2-(1H-INDOL-3-YL)ETHANIMINE | C10 H10 N2 | 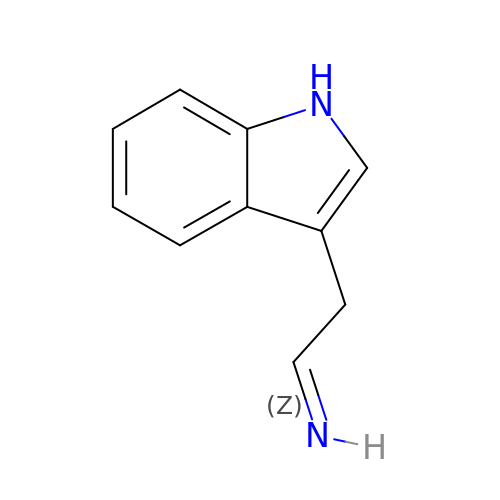DCXUMIPCJIGNQW-WDZFZDKYSA-N>EEEAEMKAVATSPSGRFLKFDIELGRGA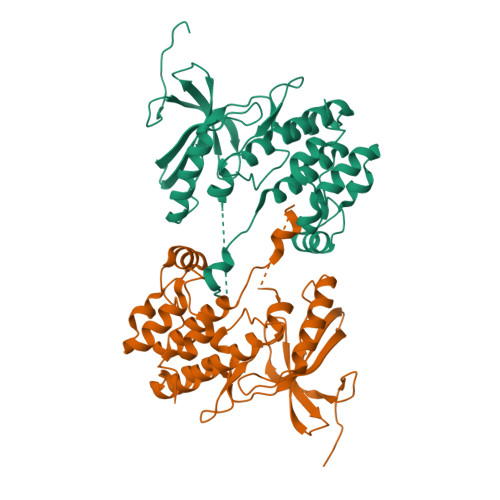FKTVYKGLDTETWVEVAWCELQDRKLTKAEQQRFKEEAEMLKGLQHPNIVRFYDSWESILKGKKCIVLVTELMTSGTLKTYLKRFKVMKPKVLRSWCRQILKGLQFLHTRTPPIIHRDLKCNNIFITGPTGSVKIGDLGLATLMRTSFAKSVIGTPAFMAPEMYEEHFDESVDVYAFGMCMLEMATSEYPYSECQNAAQIYRKVTSGIKPASFNKVTDPEVKEIIEGCIRQNKSERLSIRDLLNHAFFAEDT[2x]>MSLVVFPFKHEHPEVLLHNVRVAAAHPRVHEVLCIGYERDQTYEAVERAAPEISRATGTPVSVRLQERLGTLRPGKGDGMNTALRYFLEETQWERIHFYDADITSFGPDWITKAEEAADFGYGLVRHYFPRASTDAMITWMITRTGFALLWPHTELSWIEQPLGGELLMRREVAAMLYEDERVRRRSDWGIDTLYTFVTVQQGVSIYECYIPEGKAHRLYGGLDDLRTMLVECFAAIQSLQHEVVGQPAIHRQEHPHRVPVHIAERVGYDVEATLHRLMQHWTPRQVELLELFTTPVREGLRTCQRRPAFNFMDEMAWAATYHVLLEHFQPGDPDWEELLFKLWTTRVLNYTMTVALRGYDYAQQYLYRMLGRYRYQAALEN[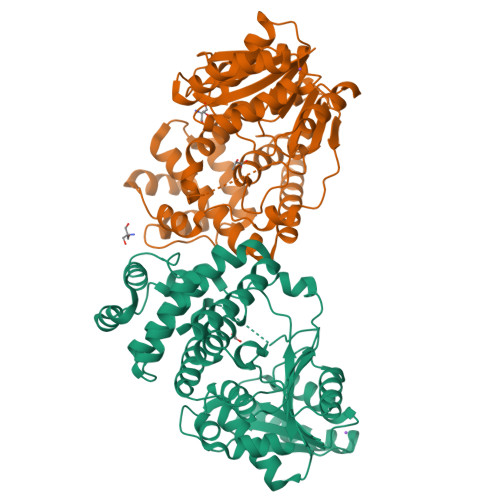2x]>MARVVVDAQAARAIGKGAMIVFKKGVVRVEGDIKPGDIVEVYTRGGKFLGKGFANPNSNIMVRIVTKDKDVEINKDLFKRRIKKANEYRKKVLKYTNVYRMVYGEADYLPGLIVDRFNDIASLQISSAGMERFKLDVAEAIMEVEPGIETVFEKNTGRSRRREGLPEIERVLLGKEKYRTIIQEGRAKFIVDMRGQKTGFFLDQRENRLALEKWVQPGDRVLDVFTYTGGFAIHAAIAGADEVIGIDKSPRAIETAKENAKLNGVEDRM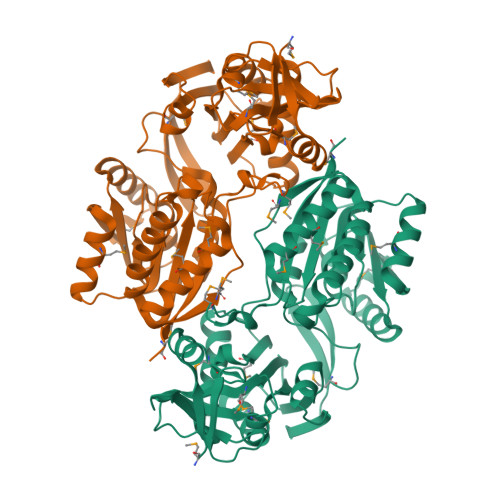KFIVGSAFEEMEKLQKKGEKFDIVVLDPPAFVQHEKDLKAGLRAYFNVNFAGLNLVKDGGILVTCSCSQHVDLQMFKDMIIAAGAKAGKFLKMLEPYRTQAPDHPILMASKDTEYLKCLFLYVEDMR[2x]> MAAQGVGPGPGSAAPPGLEAARQKLALRRKKVLSTEEMELYELAQAAGGGIDPDVFKILVDLLKLNVAPLAVFQMLKSMCAGQRLASEPQDPAAV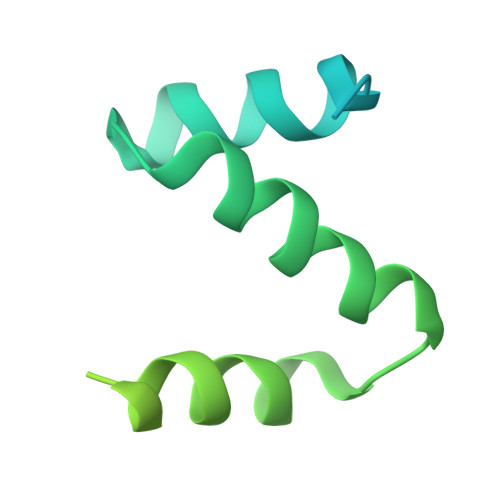SLPTSSVPETRGRDKGSAALGGVLALAERSNHEGSSQRMPRQPSATRLPKGGGPGKSPTQGST> GGAUCAUAUAAUCGCGUGGAUAUGGCACGCAAGUU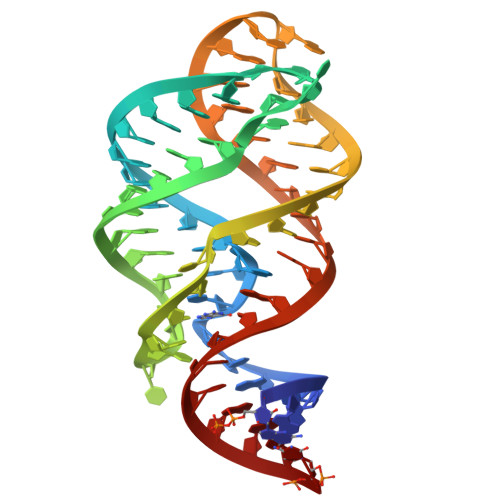UCUACCGGGCACCGUAAAUGUCCGACUAUGGUC>MASTSFLQVLIALICLVLLCERSCLASRQSSPQSITEKQGIGECDLQRVNPLEPAHRIQHEAGYSEIWDPTSRELQCAGIDATRHVIENRGLFVPSYNNAPMLIIVVQGHGILGAVFPGCPETFQSFHPTEKEGGDSRGPDQTFRDQHQKVHFIRQGDVIALPAGIVHWAYNEATEKLVLLVIHDLSNRENQLDQNLRRYFLGGNQKGDEETWAVGSKNLLWNNVFQPLDPQFLGRASGVNSEIIKKLQSENDFRGYMVRVRDGLRLVRPSSEEPRPPRPLLDNGYEETLCTVRIKENLLNPERADIYTSRGGTVSTLNSYNLPILRKLQLSANREYLYPNAMIVPEWNN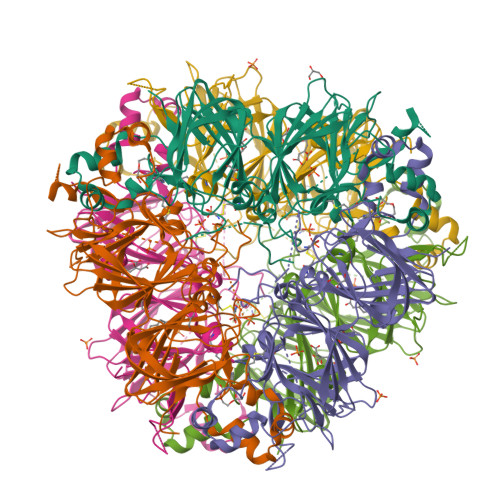NAHSISYVTRGSGRLQVGGSSKSTVYDGDVRQGQLFIIPQNYVYLKQAGPQGLELYTVKTNDRAKATALVGRTSVIRAVPLDVWINVFQLTQDEARSLKYNREEITVLDPELPKPQPEGGGYYPWSIVA[6x]4,5,6,7-tetrahydro-1-benzofuran-3-carboxylic acid | C9 H10 O3 | 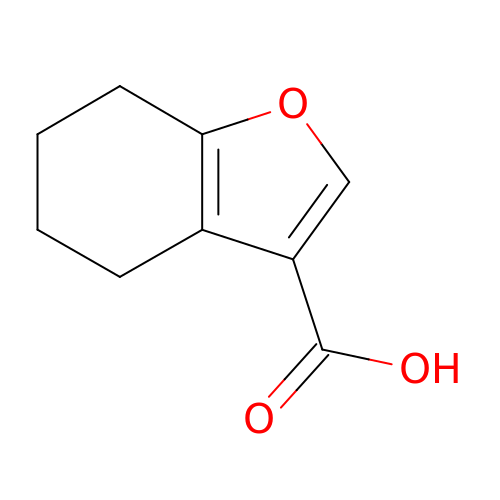QQPMDRGNNFKVEL-UHFFFAOYSA-N>MSSDADAHKVGLIPVTLMVSGNIMGSGVFLLPANLASTGGIAIYGWLVTIIGALGLSMVYAKMSFLDPSPGGSYAYARRCFGPFLGYQTNVLYWLACWIGNIAMVVIGVGYLSYFFPILKDPLVLTITCVVVLWIFVLLNIVGPKMITRVQAVATVLALIPIVGIAVFGWFWFRGETYMAAWNVSGLGTFGAIQSTLNVTLWSFIGVESASVAAGVVKNPKRNVPIATIGGVLIAAVCYVLSTTAIMGMIPNAALRVSASPFGD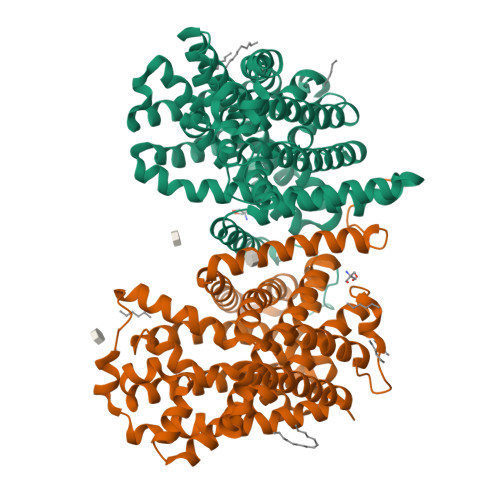AARMALGDTAGAIVSFCAAAGCLGSLGGWTLLAGQTAKAAADDGLFPPIFARVNKAGTPVAGLIIVGILMTIFQLSSISPNATKEFGLVSSVSVIFTLVPYLYTCAALLLLGHGHFGKARPAYLAVTTIAFLYCIWAVVGSGAKEVMWSFVTLMVITAMYALNYNRLHKNPYPLDAPISKDLELEVLFQ[2x]> MAGGEAGVTLGQPHLSRQDLTTLDVTKLTPLSHEVISRQATINIGTIGHVAHGKSTVVKAISGVHTVRFKNELERNITIKLGYANAKIYKLDDPSCPRPECYRSCGSSTPDE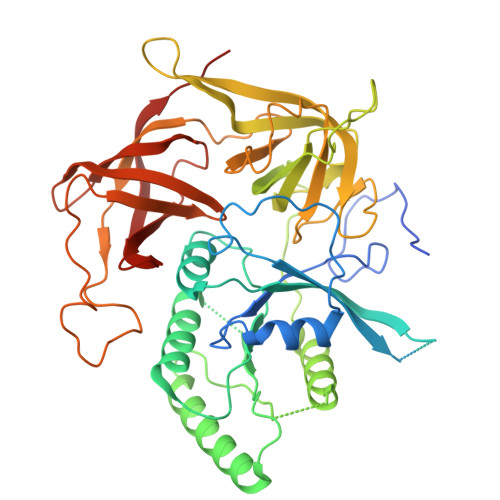FPTDIPGTKGNFKLVRHVSFVDCPGHDILMATMLNGAAVMDAALLLIAGNESCPQPQTSEHLAAIEIMKLKHILILQNKIDLVKESQAKEQYEQILAFVQGTVAEGAPIIPISAQLKYNIEVVCEYIVKKIPVPPRDFTSEPRLIVIRSFDVNKPGCEVDDLKGGVAGGSILKGVLKVGQEIEVRPGIVSKDSEGKLMCKPIFSKIVSLFAEHNDLQYAAPGGLIGVGTKIDPTLCRADRMVGQVLGAVGALPEIFTELEISYFLLRRLLGVRTEGDKKAAKVQKLSKNEVLMVNIGSLSTGGRVSAVKADLGKIVLTNPVCTEVGEKIALSRRVEKHWRLIGWGQIRRGVTIKPTVDDD> KMKKILSFDIDNTLN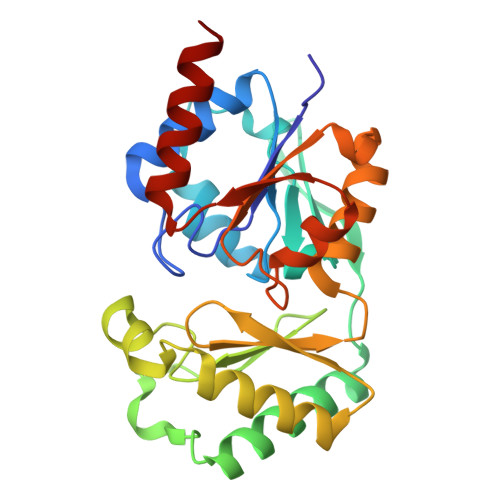EPKMPIFPEMAELLATLSQKYIIAPISGQKYDQFLIQIINNLPESANLDNFHLFVAQGTQYYAHKAGEWKQVFNYALTDEQANAIMGALEKAAKELGHWDESVLLPGDEINENRESMIAYSAIGQKAGVEAKQAWDPDMTKRNEIAKLASQYAPEFEFEVAGTTTINGFVPGQNKEFGMNHLMEELNVTKEEILYFGDMTQPGGNDYPVVQMGIETITVRDWKETAAILKAIIAMEEA>[4x]GVFTFEDEITSTVPPAKLYNAMKDADSITPKI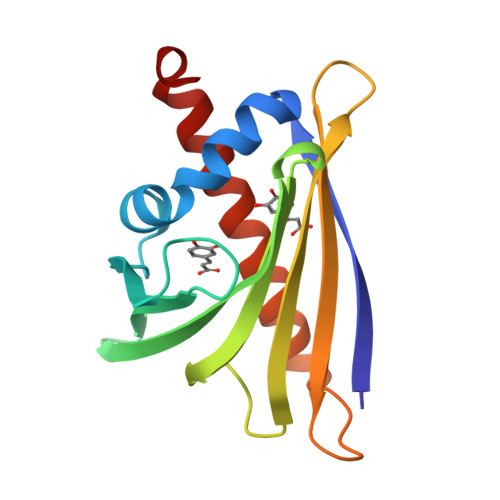IDDVKSVEIVEGNGGPGTIKKLTIVEDGETKFILHKVESIDEANYAYNYSVVGGVALPPTAEKITFETKLVEGPNGGSIGKLTLKYHTKGDAKPDEEELKKGKAKGEGLFRAIEGYVLANPTQY> MLEARLEQASILKKVVDAIKDLVQDCNFDCNDSGIALQAMDNSHVALVSMMLKTETFSPFRCDRNIALGVNLTSLTKVLRAAQNEDILTLKAEDAPDVLNLVFESSENDRISEYDLK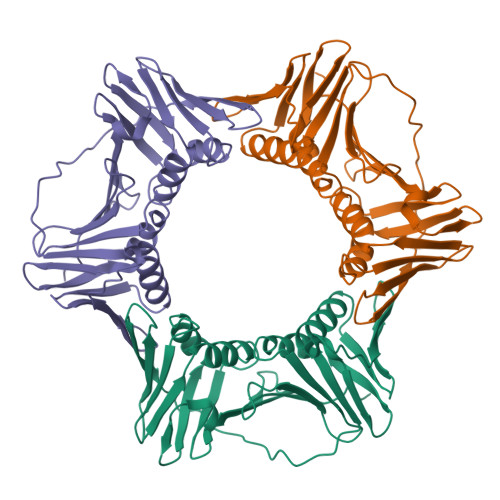LMDIDQEHLGIPDTEYAATISMPSSEFKRITTDLMAMSESVNIEASKDGVKFSCQGDIGNGSITLRQHTNVDKPSENIEIELSEPVSLTFSLKYLVNFCKASALSSTVKICLSNEVPLLVEYNISASSYLRFYLAPKIG>[2x]M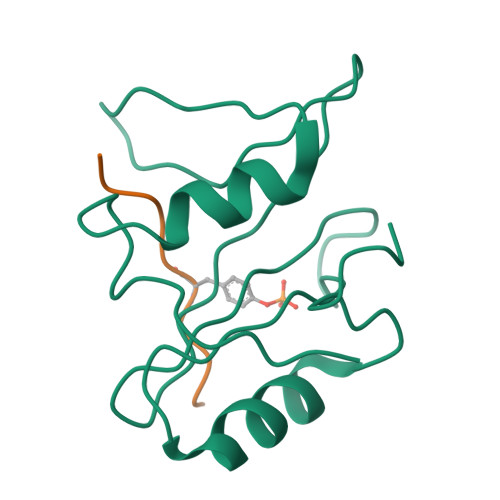DAVAVYHGKISRETGEKLLLATGLDGSYLLRDSESVPGVYCLCVLYHGYIYTYRVSQTETGSWSAETAPGVHKRYFRKIKNLISAFQKPDQGIVIPLQYPVEK;>[2x]KSLTIYAQVQK> SAKKNEPRFKNGIVAALAGFFILGIGTVGTLWILNSPQRQAAELDSLLGQEKERFQVLPGRDKMLYVAAQNER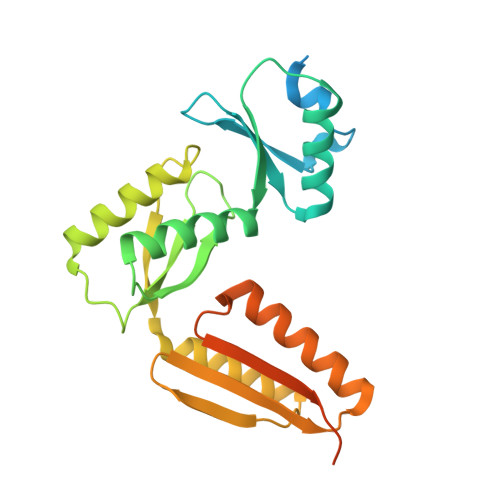DTLWARQVLARGDYDKNARVINENEENKRISIWLDTYYPQLAYYRIHFDEPRKPVFWLSRQRNTMSKKELEVLSQKLRALMPYADSVNITLMDDVTAAGQAEAGLKQQALPYSRRNHKGGVTFVIQGALDDVEILRARQFVDSYYRTWGGRYVQFAIELKDDWLKGRSFQYGAEGYIKMSPGHWYFPSPL Deregulation or mutation of DNA-binding proteins, such as transcription factors, is closely associated with the pathogenesis of several human diseases, including cancer, making them attractive therapeutic targets. Here, the structure of the DNA-binding domain (DBD) of interferon regulatory factor 4 (IRF4) bound to its interferon-stimulated response element (ISRE), solved by the use of native intrinsic phosphorus and sulfur single-wavelength anomalous dispersion methods at I23, is presented. The structure shows the presence of three molecules of the IRF4 DBD bound to one molecule of DNA, which is unexpected in the light of previous studies suggesting the homodimerization of IRF4 on ISRE elements.

The human IRF4 DBD domain was expressed, purified and co-crystallized with 21-mer DNA with an AT 5′ overhang containing an ISRE element. Taking advantage of the dedicated long-wavelength beamline I23 at Diamond Light Source, data were collected at a wavelength of 2.7552 Å with the aim of solving the structure of the complex de novo using native intrinsic phosphorus and sulfur SAD methods. The final high-multiplicity (∼80) data set to a resolution of 2.6 Å (space group C2221, unit-cell parameters a = 77.9, b = 112.4, c = 140.7 Å) was obtained by merging eight data sets collected from two crystals: four data sets from each crystal. The final model contained three molecules of the IRF4 DBD bound to one ISRE element, which fits well in the crystallo­graphic asymmetric unit (V M = 2.5 Å3 Da−1, solvent content 51%) based on an estimated molecular mass of ∼61 kDa. When calculating phased anomalous difference maps with ANODE, the three IRF4 DBD sulfur sites gave anomalous peaks that were stronger on average than the DNA phosphorus sites (∼11σ versus ∼9σ); however, one of the sulfur sites had a much lower peak height when compared with the other two sites (∼4σ compared with ∼18σ and 13σ). A further advantage of solving the phosphorus substructure was that the DNA double helix was readily recognisable and the electron-density map for the nucleic acid portion of the structure was strong. The phosphorus sites were used as well defined guides for fitting and building the DNA double-helix model, which is important when, as in this case, the DNA departs from the canonical B form. The molecular-replacement procedure was confounded by the unexpected oligomerization state of the complex: a heterotetramer with three IRF4 DBD molecules bound to one ISRE element.

>MGSHHHHHHSAALEVLFQGPGGNGKLRQWLIDQIDSGKYPGLVWENEEKSIFRIPWKHAGKQDYNREEDAALFKAWALFKGKFREGIDKPDPPTWKTRLRCALNKSNDFEELVERSQLDISDPYKVYRIVPEGAKKGAKQL[3x]>GSHN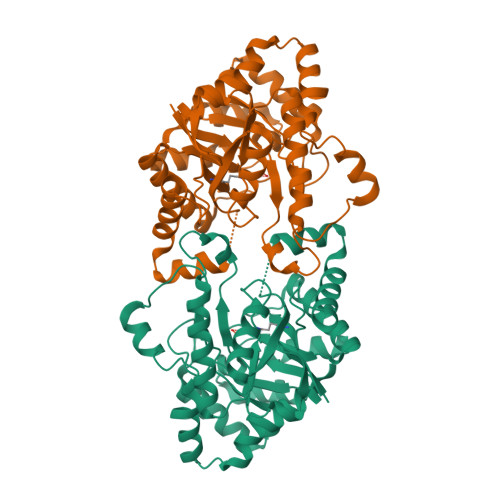MAEMVETVCGPVPVEQLGKTLIHEHFLFGYPGFQGDVTRGTFREDESLRVAVEAAEKMKRHGIQTVVDPTPNDCGRNPAFLRRVAEETGLNIICATGYYYGGEGAPPYFQFRRLLGTAEDDIYDMFMAELTEGIADTGIKAGVIKLASSKGRITEYEKMFFRAAARAQKETGAVIITHTQEGTMGPEQAAYLLEHGADPKKIVIGHMCGNTDPDYHRKTLAYGVYIAFDCFGIQGMVGAPTDEERVRTLLALLRDGYEKQIMLSHDTVNVWLGRPFTLPEPFAEMMKNWHVEHLFVNIIPALKNEGIRDEVLEQMFIGNPAALFSA[2x]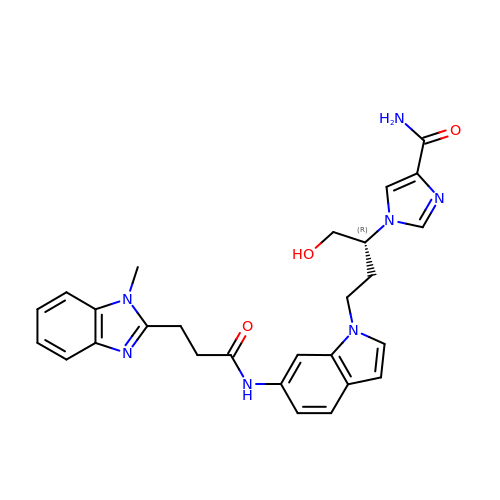1-((1R)-1-(HYDROXYMETHYL)-3-(6-((3-(1-METHYL-1H-BENZIMIDAZOL-2-YL)PROPANOYL)AMINO)-1H-INDOL-1-YL)PROPYL)-1H-IMIDAZOLE-4-CARBOXAMIDE | C27 H29 N7 O3 | MBHAURHGCAJBCN-HXUWFJFHSA-N> MLPLTLLNATQGRPILVELKNGETFNGHLENCDNYMNLTLREVIRTMPDGDKFFRLPECYIRGNNIKYLRIQDEVLSQVAKQQA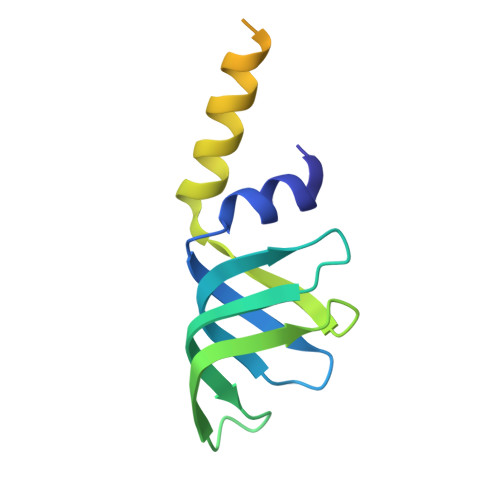QQRENRGSRFRGRGQRGRGNYGHTAPNRRGRGRGGHMWSHPQFEK> DYKDDDAMPSKSLSNLSVTTGANESGSVPEGWERDFLPASDGTTTELVIRCVIPSLYLLIITVGLLGNIMLVKIFITNSAMRSVPNIFISNLAAGDLLLLLTCVPVDASRYFFDEWMFGKVGCKLIPVI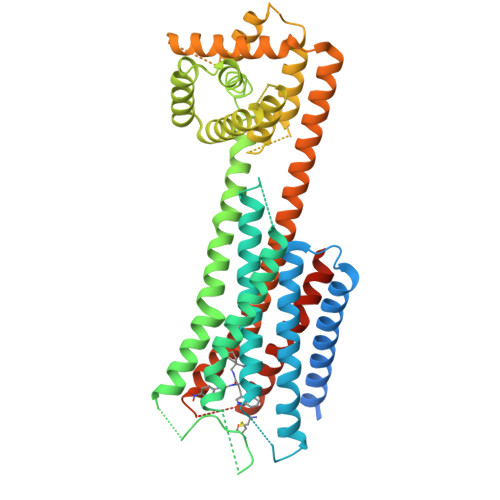QLTSVGVSVWTLTALSADRYRAIVNPMDMQTSGALLRTCVKAMGIWVVSVLLAVPEAVFSEVARISSLDNSSFTACIPYPQTDELHPKIHSVLIFLVYFLIPLAIISIYYYHIAKHLKEKAKAGAEIAAHPDAFLFLLFAAFGVVLTGDPEDRALWAELLALVERAAPGIARALAAAYRAAEEAYRAGGPVAGFRAGILGACAGVDAETRLPLTARIVDLLRTIRALRDDEAALRALVDALGAELRALLAPVAADAEELDALLARLADLALVALRELAKLSESEMDAFIADLTAAVEAMAKQMETRKRLAKIVLVFVGCFIFCWFPNHILYMYRSFNYNEIDPSLGHMIVTLVARVLSFGNSCVNPFALYLLSESFRRHFNSQLCHHHHHH> SSQKKKKIAVMTSGGDSPGMNAAVRAVVRTGIHFGCDVFAVYEGYEGLLRGGKYLKKMAWEDVRGWLSEGGTLIGTARSMEFRKREGRRQAAGNLISQGIDALVVCGGDGSLTGADLFRHEWPSLVDELVAEGRFTKEEVAPYKNLSIVGLVGSIDNDMSGTDSTIGAYSALERICEMVDYIDATAKSHSRAFVVEVMGRHCGWLALMAGIATGADYIFIPERAVPHGKWQDELKEVCQRHRSKGRRNNTIIVAEGALDDQLNPVTANDVKDALIELGLDTKVTILGHVQRGGTAVAHDRWLATLQGVDAVKAVLEFTPETPSPLIGILENKIIRMPLVESVKLTKSVATAIENKDFDKAISLRDTEFIELYENFLSTTVKDDGSELLPVSDRLNIGIVHVGAPSAALNAATRAATLYCLSHGHKPYAIMNGFSGLIQTGEVKELSWIDVENWHNLGGSEIGTNRSVASEDLGTIAYYFQKNKLDGLIILGGFEGFRSLKQLRDGRTQHPIFNIPMCLIPATVSNNVPGTEYSLGVDTCLNALVNYTDDIKQSASATRRRVFVCEVQGGHSGYIASFTGLITGAVSVYTPEKKIDLASIREDITLLKENFRHDKGENRN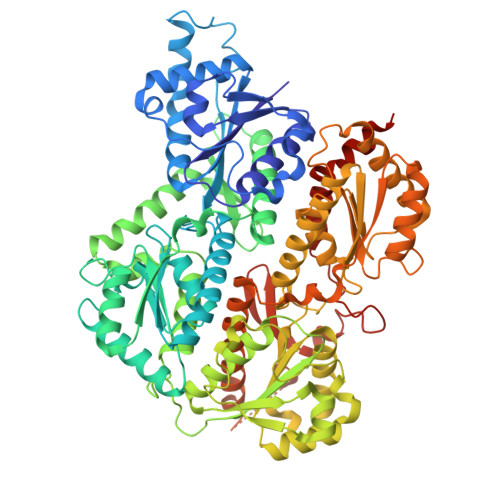GKLLVRNEQASSVYSTQLLADIISEASKGKFGVRTAIPGHVQQGGVPSSKDRVTASRFAVKCIKFIEQWNKKNEASPNTDAKVLRFKFDTHGEKVPTVEHEDDSAAVICVNGSHVSFKPIANLWENETNVELRKGFEVHWAEYNKIGDILSGRLKLRAEVAALAAENK> MENSARQVAQDTRELHLLQHIKSDQSYIYVFVFLYYRDHSVRVWKLTNPVSISETLDYDDLINNVNRCKSAREPAIYYREGITGNDAGDSIIDKAYCEPVSFMIVACGDVDIQTIEVNIQGYDEIEGVGILDSNVTPPYAITATKFERKTSGGYIFYTYCGLFGHGDRGHPTMAVGVEKKNRNAFGRMHPMYVAANYKRRNFWAKKDWWFPTEGQMVEQFIKQQSIPYVTADNVMIAPCVREIRHHAHY

Cypoviruses, members of the family Reoviridae, subfamily Spinareovirus, possess a single capsid layer with turrets and are commonly embedded in crystalline occlusion bodies called polyhedra, which are formed in the cell cytoplasm and mainly composed of a single virus-encoded protein, polyhedrin. To ensure the delivery of virus particles to the target intestinal cells, allowing the transmission of packages of infectious virus between hosts by oral-faecal routes, polyhedra are disrupted only when they are exposed to the very alkaline pH environment found in insect midguts. The fold of all the polyhedrins is highly similar – a β-barrel core sitting on a base domain, surrounded by a common array of five helices (H1–H5). The strongest intermolecular interactions define a trimer composed of a cluster of three β-barrels sandwiched by helices top and bottom.

CPV14 essentially lacks a V1 extension whereas a long V5 loop forms a hook and an intra-molecular disulphide bridge helps to stabilise the base domain. The full length polyhedrin structures are generally well ordered, as expected for a crystal lattice which has extensive interactions and low solvent content (19–25%), however some types show regions of flexibility: 13 residues (136–148) of CPV5 and 6 residues (68–73) of CPV14 have high (>40 compared with an overall Wilson B-factor of 21.3) B-factors, whilst 13 residues (66–78) of CPV15 could not be modelled. These areas are in structurally variable parts of the proteins. In CPV14, a GTP is located ∼5 Å from the CPV1 position, in a different conformation, binding to the backbone of V2c and embraced by V1 and bulky side chains of an elongated V5. A change in the conformation of the V4 hairpin switches it to bind another monomer. In CPV14 and CPV19 the V2n loops move to occupy some of the central space. In CPV1, 14, 15, 17, 18 and 20 solvent molecules can move between these two voids, whereas in CPV4, 5 and 19 they are blocked by tyrosine residues.> MAESASPPSSSAAAPAAEPGVTTEQPGPRSPPSSPPGLEEPLDGADPHVPHPDLAPIAFFCLRQTTSPRNWCIKMVCN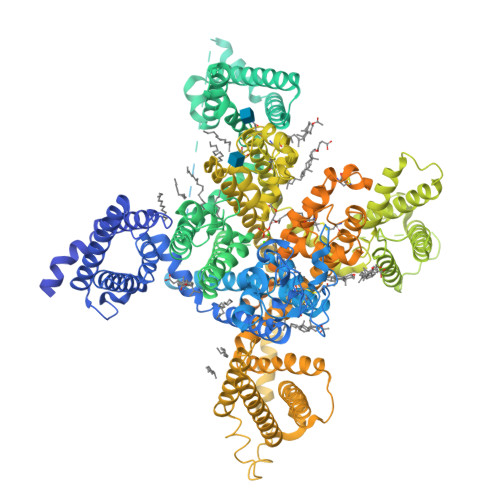PWFECVSMLVILLNCVTLGMYQPCDDMDCLSDRCKILQVFDDFIFIFFAMEMVLKMVALGIFGKKCYLGDTWNRLDFFIVMAGMVEYSLDLQNINLSAIRTVRVLRPLKAINRVPSMRILVNLLLDTLPMLGNVLLLCFFVFFIFGIIGVQLWAGLLRNRCFLEENFTIQGDVALPPYYQPEEDDEMPFICSLSGDNGIMGCHEIPPLKEQGRECCLSKDDVYDFGAGRQDLNASGLCVNWNRYYNVCRTGSANPHKGAINFDNIGYAWIVIFQVITLEGWVEIMYYVMDAHSFYNFIYFILLIIVGSFFMINLCLVVIATQFSETKQREHRLMLEQRQRYLSSSTVASYAEPGDCYEEIFQYVCHILRKAKRRALGLYQALQSRRQALGPEAPAPAKPGPHAKEPRHYHGKTKGQGDEGRHLGSRHCQTLHGPASPGNDHSGRELCPQHSPLDATPHTLVQPIPATLASDPASCPCCQHEDGRRPSGLGSTDSGQEGSGSGSSAGGEDEADGDGARSSEDGASSELGKEEEEEEQADGAVWLCGDVWRETRAKLRGIVDSKYFNRGIMMAILVNTVSMGIEHHEQPEELTNILEICNVVFTSMFALEMILKLAAFGLFDYLRNPYNIFDSIIVIISIWEIVGQADGGLSVLRTFRLLRVLKLVRFMPALRRQLVVLMKTMDNVATFCMLLMLFIFIFSILGMHIFGCKFSLRTDTGDTVPDRKNFDSLLWAIVTVFQILTQEDWNVVLYNGMASTSPWASLYFVALMTFGNYVLFNLLVAILVEGFQAEGDANRSYSDEDQSSSNIEEFDKLQEGLDSSGDPKLCPIPMTPNGHLDPSLPLGGHLGPAGAAGPAPRLSLQPDPMLVALGSRKSSVMSLGRMSYDQRSLSSSRSSYYGPWGRSAAWASRRSSWNSLKHKPPSAEHESLLSAERGGGARVCEVAADEGPPRAAPLHTPHAHHIHHGPHLAHRHRHHRRTLSLDNRDSVDLAELVPAVGAHPRAAWRAAGPAPGHEDCNGRMPSIAKDVFTKMGDRGDRGEDEEEIDYTLCFRVRKMIDVYKPDWCEVREDWSVYLFSPENRFRVLCQTIIAHKLFDYVVLAFIFLNCITIALERPQIEAGSTERIFLTVSNYIFTAIFVGEMTLKVVSLGLYFGEQAYLRSSWNVLDGFLVFVSIIDIVVSLASAGGAKILGVLRVLRLLRTLRPLRVISRAPGLKLVVETLISSLKPIGNIVLICCAFFIIFGILGVQLFKGKFYHCLGVDTRNITNRSDCMAANYRWVHHKYNFDNLGQALMSLFVLASKDGWVNIMYNGLDAVAVDQQPVTNHNPWMLLYFISFLLIVSFFVLNMFVGVVVENFHKCRQHQEAEEARRREEKRLRRLEKKRRKAQRLPYYATYCHTRLLIHSMCTSHYLDIFITFIICLNVVTMSLEHYNQPTSLETALKYCNYMFTTVFVLEAVLKLVAFGLRRFFKDRWNQLDLAIVLLSVMGITLEEIEINAALPINPTIIRIMRVLRIARVLKLLKMATGMRALLDTVVQALPQVGNLGLLFMLLFFIYAALGVELFGKLVCNDENPCEGMSRHATFENFGMAFLTLFQVSTGDNWNGIMKDTLRDCTHDERSCLSSLQFVSPLYFVSFVLTAQFVLINVVVAVLMKHLDDSNKEAQEDAEMDAELELEMAHGLGPGPRLPTGSPGAPGRGPGGAGGGGDTEGGLCRRCYSPAQENLWLDSVSLIIKDSLEGELTIIDNLSGSIFHHYSSPAGCKKCHHDKQEVQLAETEAFSLNSDRSSSILLGDDLSLEDPTACPPGRKDSKGELDPPEPMRVGDLGECFFPLSSTAVSPDPENFLCEMEEIPFNPVRSWLKHDSSQAPPSPFSPDASSPLLPMPAEFFHPAVSASQKGPEKGTGTGTLPKIALQGSWASLRSPRVNCTLLRQATGSDTSLDASPSSSAGSLQTTLEDSLTLSDSPRRALGPPAPAPGPRAGLSPAARRRLSLRGRGLFSLRGLRAHQRSHSSGGSTSPGCTHHDSMDPSDEEGRGGAGGGGAGSEHSETLSSLSLTSLFCPPPPPPAPGLTPARKFSSTSSLAAPGRPHAAALAHGLARSPSWAADRSKDPPGRAPLPMGLGPLAPPPQPLPGELEPGDAASKRKR> G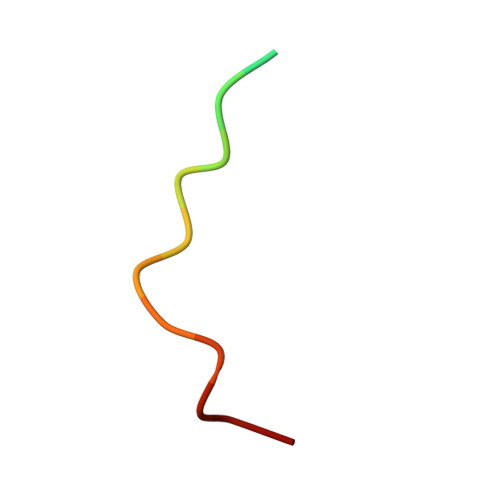PETLVCHEVDLDDL>[2x]MGSMHAALSTEVVHLRQRTEELLRCNEQQAAELETCKEQLFQSNMERKELHNTVMDLRGNIRVFCRIRPPLESEENRMCCTWTYHDESTVELQSIDAQAKSKMGQQIFSFDQVFHPLSSQSDIFEMVSPLIQSALDGYNICIFAYGQTGSGKTYTMDGVPESVGVIPRTVDLLFDSIRGYRNLGWEYEIKATFLEIYNEVLYDLLSNEQKDMEIRMAKNNKNDI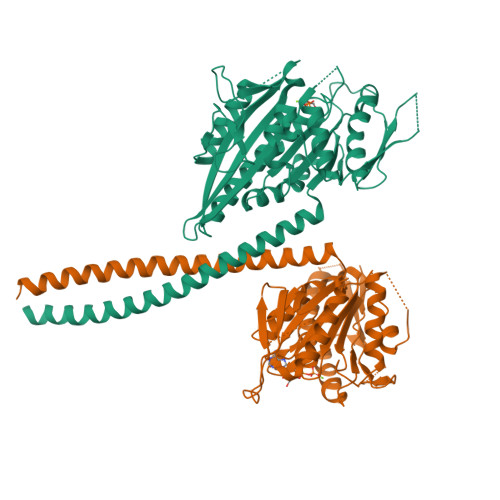YVSNITEETVLDPNHLRHLMHTAKMNRATASTAGNERSSRSHAVTKLELIGRHAEKQEISVGSINLVDLAGSESPKTSTRMTETKNINRSLSELTNVILALLQKQDHIPYRNSKLTHLLMPSLGGNSKTLMFINVSPFQDCFQESVKSLRFAASVNSCKMTKAKRNRYLNNSVANSSTQSNNSGNFDK>MGHHHHHHHHHHSSGHIDDDKHMGGYSMHQLQGNKEYGSEKKGFLLKKSDGIRKVW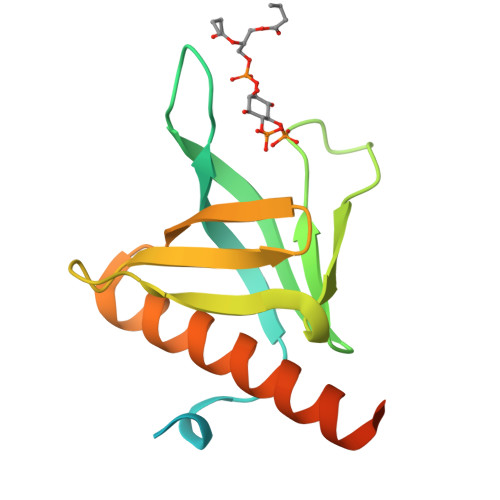QRRKCAVKNGILTISHATSNRQPAKLNLLTCQVKPNAEDKKSFDLISHNRTYHFQAEDEQDYIAWISVLTNSKEEALTMAFRGEQSTGENSLED[2x]> MTQKMDFDAIIIGAGFGGLYSLKKLRDDFNLKVRAFDRATEVGGTWFWNQYPGALSDSETHLYCYSWDKELLQEMEIKRKYISQPDVLAYLKRVADKHDLRKDIQF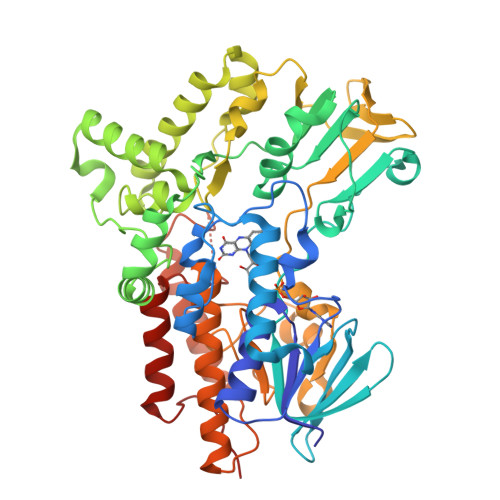ETGIRSAYFDEENSFWNVTTENDEKFTARFLITALGLLAAPNLPKIKGIETFKGELHHTSRWPKDVTFSGKRVGVIGTGSTGVQVITAIASQVKHLTVFQRSAQYSVPIGNVVMSETDVAKIKENYDQIWENVWNSALGYGLNESTLPTMSVSAEERDKIFEKAWQEGGGFRFMFETFGDIAVDETANIEAQNFIKKKISEIVKDPFVAKKLTPTDLYACRPLCDSGYYEIFNRDNVSLEDVKANPIVEIKEDCVVTADGVEHKLDMLICATGFDAVDGSYKRIDIRGKDGISIKDHWKDGPNSYLGMMVSNFPNMFMVFGPNGPVANSPPIIETQVRWIADLIGYAEDHQINQIEATKDAVDNWTNTCSDIANKTLFAKAKCRIFGANVPGKKNTVYLYMGGLKEYRNQISEVSNNNYKGCLLKQ> XNPE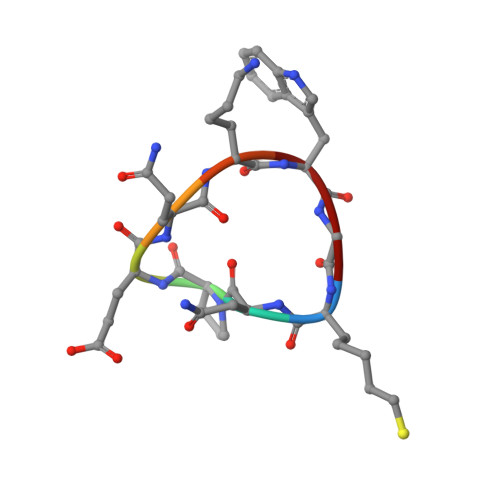QKWG>MASVKLKGVYKRYPGGVTAVNDFNLDIEDKEFIILVGPSGCGKTTTLRMVAGLEEITEGELYIGDKLVNDVAPKDRDIAMVFQNYALYPHMSVFDNMAFGLKLRKVPKDEIKRRVLEAAKILDIEHLLERKPKALSGGQRQRVALGRAIVRNPKVFLMDEPLSNLDAKLRVQMRTEISKLHQRLQTTFIYVTHDQTEALTMGTRIVVMKDGYIQQVDTPTNLYERPCNMFVAGFIGSPQMNFVNARIEKRGDEMHLLFGKQDIKLPEGKAKKLESSEYVGREVVMGIRPENIRDEEIYLESMSENVVEGRVEVVEMLGSETLIYMVIDDFEFTARVNPRSKARPGDVIKVAFDANKIHLFDKETEKTIMN[2x]

Clostridium thermocellum has extensive potential in lignocellulose biorefineries as an environmentally prominent, thermophilic, cellulolytic bacterium. Previously, five putative sugar transporters, denoted A to D and L and belonging to the ABC transport systems group, were identified in the genome of C. thermocellum, and the solute-binding lipoproteins (SBP) of these ABC transporters were shown to bind different dextrins by isothermal titration calorimetry (ITC) assays. To gain insight into the structural mechanism of the transporter specificities, 11 crystal structures, both alone and in complex with appropriate saccharides, were solved for all 5 putative sugar-binding proteins, thus providing detailed specific interactions between the proteins and the corresponding saccharides. Combined genetic, biophysical, and structural studies have provided solid evidence that transporter A and transporter B are the major glucose and cellodextrin transporters, respectively, among the five potential sugar transporters in C. thermocellum.

Considering the importance of transporter B as the major cellodextrin transporter, we further identified its cryptic, hitherto unknown ATPase-encoding gene as clo1313_2554, which is located outside the transporter B gene cluster. We therefore suspected that Clo1313_2554 represents the ATPase subunit of transporter B. Therefore, we deleted clo1313_2554 using homologous recombination and obtained the Δ2554 mutant. The Δ2554 mutant lost the ability to grow on cellobiose and Avicel, in a manner similar to that of the ΔtransporterB strain. Therefore, the same phenotypes of the Δ2554 and ΔtransporterB mutants imply that Clo1313_2554 is the missing ATPase subunit of transporter B, which is the sole cellodextrin transporter in C. thermocellum. To better confirm the function of Clo1313_2554, the crystal structure of Clo1313_2554 was determined at 2.8 Å resolution. Clo1313_2554 presents the general α/β-type ATPase domain fold in homodimer form, similar to that of other NBD crystal structures. The ATP-binding Walker A motif from subunit A and the ABC signature motif from subunit B were approximately 30 Å apart in the structure, indicating that the nucleotide-free homodimer was in an open conformation. The crystal structure of the ATPase was solved, showing that it represents a typical nucleotide-binding domain of the ATP-binding cassette (ABC) transporter. The ATPase subunit of transporter B was identified as the encoded product of clo1313_2554, which is located outside the gene cluster of transporter B. Interestingly, this feature is found in many other bacteria.>[2x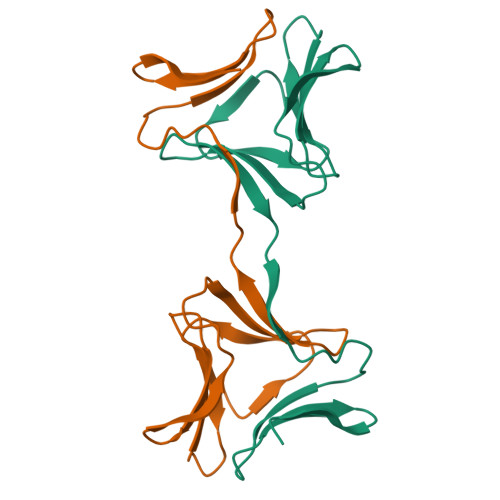]MGDTLTAGQKLERGGSLQSGNGAYTLTLQDDGNLVLYARDKAVWSTGTNGQDVVRAEVQTDGNFVLYTAEKPVWHTDTKGKKEVKLVLQDDRNLVLYAKDGPAWSLEHHHHHH> GPHMMSRGQTEGSQAMASSQAAGPGPSP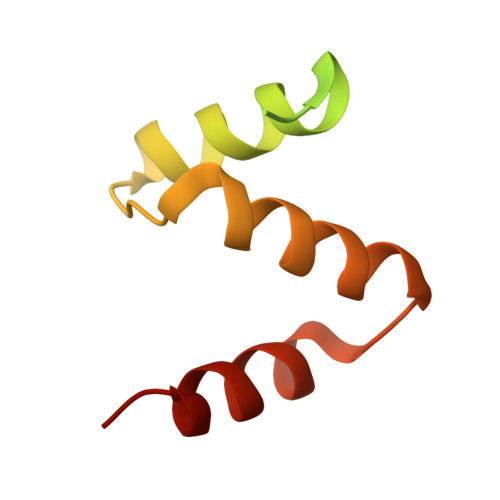DAIVSVSGTVQKYVAKKKKVLNPEEAELYELTQAAGIVIDQEVFKILVDLLKMNVAPLAVFQMLKSMCAG>[2x]AELVSDKALESAPTVGWASQNGFTTGGAAATSDNIYIVTNISEFTSALSAGAEAKIIQIKGTIDISGGTPYTDFADQKA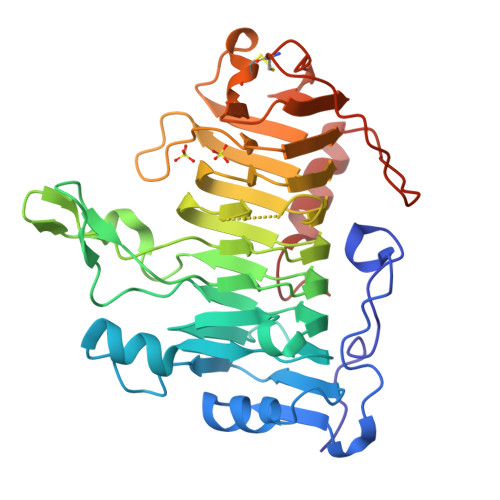RSQINIPANTTVIGLGTDAKFINGSLIIDGTDGTNNVIIRNVYIQTPIDVEPHYEKGDGWNAEWDAMNITNGAHHVWIDHVTISDGNFTDDMYTTKDGETYVQHDGALDIKRGSDYVTISNSLIDQHDKTMLIGHNDTNSAQDKGKLHVTLFNNVFNRVTERAPRVRYGSIHSFNNVFKGDAKDPVYRYQYSFGIGTSGSVLSEGNSFTIANLSASKACKVVKKFNGSIFSDNGSVLNGSAVDLSGCGFSAYTSKIPYIYDVQPMTTELAQSITDNAGSGKL N-(2-amino-2-oxoethyl)-5'-[(4aR,8aS)-3-cycloheptyl-4-oxo-3,4,4a,5,8,8a-hexahydrophthalazin-1-yl]-2'-methoxy[1,1'-biphenyl]-4-carboxamide | C31 H36 N4 O4 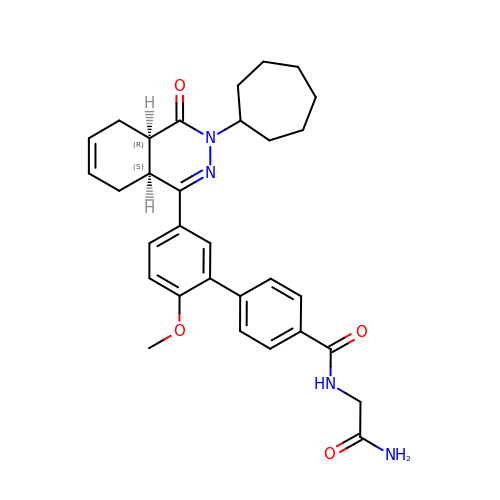| VZKJWTFPORBEEH-LOSJGSFVSA-N>MRILKIYENKGVYKVVIGEPFPPIEFPLEQKISSNKSLSELGLTIVQQGNKVIVEKSLDLKEHIIGLGEKAFELDRKRKRYVMYNVDAGAYKKYQDPLYVSIPLFISVKDGVATGYFFNSASKVIFDVGLEEYDKVIVTIPEDSVEFYVIEGPRIEDVLEKYTELTGKPFLPPMWAFGYMISRYSYYPQDKVVELVDIMQKEGFRVAGVFLDIHYMDSYKLFTWHPYRFPEPKKLIDELHKRNVKLITIVDHGIRVDQNYSPFLSGMGKFCEIESGELFVGKMWPGTTVYPDFFREDTREWWAGLISEWLSQGVDGIWLDMNEPTDFSRAIEIRDVLSSLPVQFRDDRLVTTFPDNVVHYLRGKRVKHEKVRNAYPLYEAMATFKGFRTSHRNEIFILSRAGYAGIQRYAFIWTGDNTPSWDDLKLQLQLVLGLSISGVPFVGCDIGGFQGRNFAEIDNSMDLLVKYYALALFFPFYRSHKATDGIDTEPVFLPDYYKEKVKEIVELRYKFLPYIYSLALEASEKGHPVIRPLFYEFQDDDDMYRIEDEYMVGKYLLYAPIVSKEESRLVTLPRGKWYN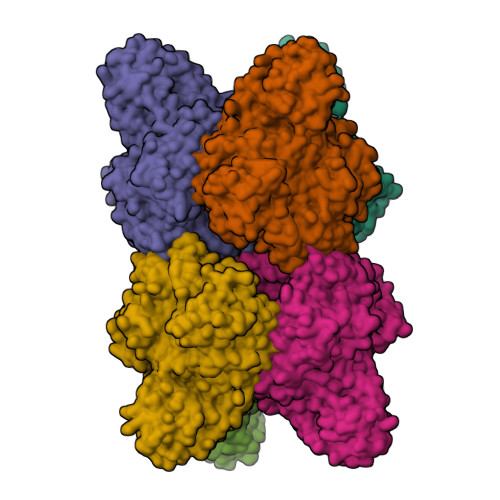YWNGEIINGKSVVKSTHELPIYLREGSIIPLEGDELIVYGETSFKRYDNAEITSSSNEIKFSREIYVSKLTITSEKPVSKIIVDDSKEIQVEKTMQNTYVAKINQKIRGKINLE[6x]> MHRDAWLPRPAFSLTGLSLFFSLVPPGRSMEVTVPATLNVLNGSDARLPCTFNSCYTVNHKQFSLNWTYQECNNCSEEMFLQFRMKIINLKLERFQDRVEFSGNPSKYDVSVMLRNVQPEDEGIYNCYIMNPPDRHRGHGKIHLQVLMEEPPERDSTVAVIVGASVGGF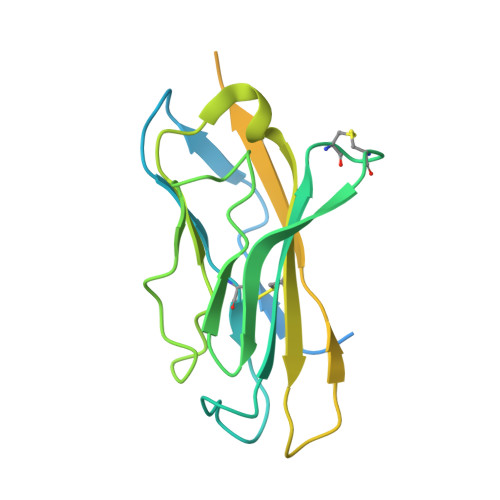LAVVILVLMVVKCVRRKKEQKLSTDDLKTEEEGKTDGEGNPDDGAK>[12x]MRDSNNIKYVREDAKKMHKLWAHIRMAMEGSRAIKDNAKEFVPHPDNTKATTPEGVARYKAYIERAVWYGASANTVDGMLGQI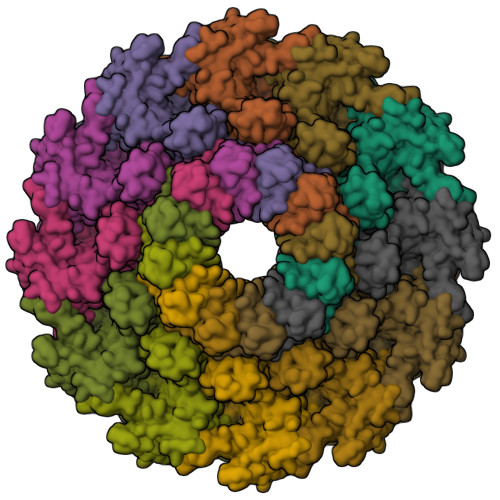FARDPVFTGPEDKFDMLINDVDGSGLSIHQQARDSAEDALSLGRGGLFVDYSYVTTNGVSEAQEESGEARPYIKFIAAEDILNWRERWVNGAKRTTLLVFREESDADDDGYQIYKEEVWRELRLVDGTYWQRTWRENDGQLYVDDWISPTKADGSQFDEIPFVIFGSKNNDPTIDMPPMRDLVELNIAHFRNSADYEEACFICGQPTLFLSGLTEHWVKNVLGGAVVIGSRDAVPLPVNAKPELLQAEGNGMVKEAMDQKERQMVALGAKLIDSDKTQRTFGEASMEAAAQNSVLSRVSKNVSDAYTKALRWAAMFLGLDEKIEYELNSDFDINKMSPEELAAVISAWQSNAISFTEMRWQIKKGGRAYLEDEDMRNESEQDDPLKLDITKPDPNEDPNASEDDQTDPNDETKEKDAETGGAE(3S)-1-(2-hydroxyphenyl)-5-oxopyrrolidine-3-carboxylic acid | C11 H11 N O4 | 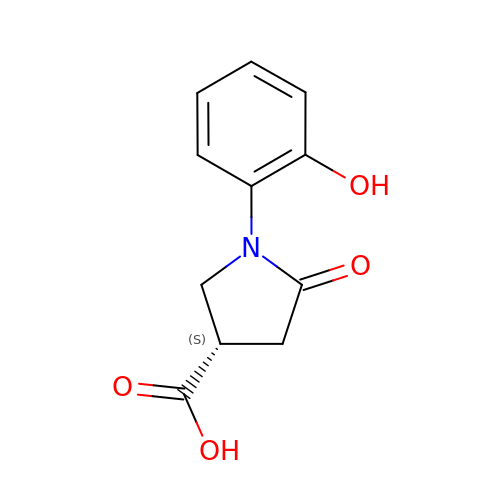FPQOSKXLHCTVED-ZETCQYMHSA-N>[2x]SAKDPWEQTLKANDLEVKIKSV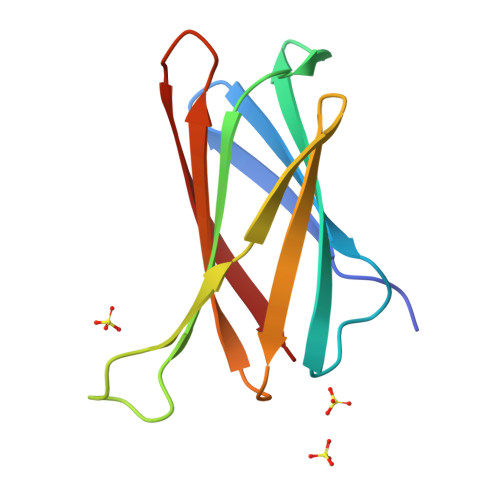GNPIKGDNTFVLSPTLKGKALEKAIVRVQFMMPEMPGMPAMKEMAQVSEKNGLYEAKTNLSMNGTWQVRVDIKSKEGEVYRAKTSLDL> GP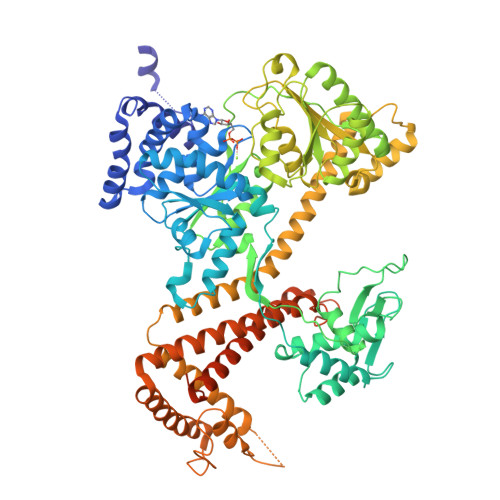HMLGILNKMFDPTKRTLNRYEKIANDIDAIRGDYENLSDDALKHKTIEFKERLEKGATTDDLLVEAFAVVREASRRVTGMFPFKVQLMGGVALHDGNIAEMKTGEGKTLTSTLPVYLNALTGKGVHVVTVNEYLASRDAEQMGKIFEFLGLTVGLNLNSMSKDEKREAYAADITYSTNNELGFDYLRDNMVLYKEQMVQRPLHFAVIDEVDSILIDEARTPLIISGQAAKSTKLYVQANAFVRTLKAEKDYTYDIKTKAVQLTEEGMTKAEKAFGIDNLFDVKHVALNHHINQALKAHVAMQKDVDYVVEDGQVVIVDSFTGRLMKGRRYSEGLHQAIEAKEGLEIQNESMTLATITFQNYFRMYEKLAGMTGTAKTEEEEFRNIYNMQVVTIPTNRPVVRDDRPDLIYRTMEGKFKAVAEDVAQRYMTGQPVLVGTVAVETSELISKLLKNKGIPHQVLNAKNHEREAQIIEEAGQKGAVTIATNMAGRGTDIKLGEGVKELGGLAVVGTERHESRRIDNQLRGRSGRQGDPGITQFYLSMEDELMRRFGAERTMAMLDRFGMDDSTPIQSKMVSRAVESSQKRVEGNNFDSRKQLLQYDDVLRQQREVIYKQRFEVIDSENLREIVENMIKSSLERAIAAYTPREELPEEWKLDGLVDLINTTYLDEGALEKSDIFGKEPDEMLELIMDRIITKYNEKEEQFGKEQMREFEKVIVLRAVDSKWMDHIDAMDQLRQGIHLRAYAQTNPLREYQMEGFAMFEHMIESIEDEVAKFVMKAEIENNLEREEVVQGQTTAHQPQEGDDNKKAKKAPVRKVVDIGRNAPCHCGSGKKYKNCCGRTE> MATGTRYAGKVVVVTGGGRGIGAGIVRAFVNSGARVVICDKDESGGRALEQEL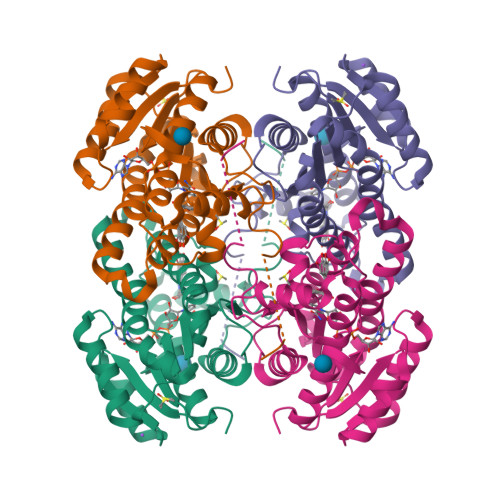PGAVFILCDVTQEDDVKTLVSETIRRFGRLDCVVNNAGHHPPPQRPEETSAQGFRQLLELNLLGTYTLTKLALPYLRKSQGNVINISSLVGAIGQAQAVPYVATKGAVTAMTKALALDESPYGVRVNCISPGNIWTPLWEELAALMPDPRASIREGMLAQPLGRMGQPAEVGAAAVFLASEANFCTGIELLVTGGAELGAGCKASRSTPVDAPDIPS>GAMVDKGFINIFPMINTTVFVNDGENVDLIVEYEAFP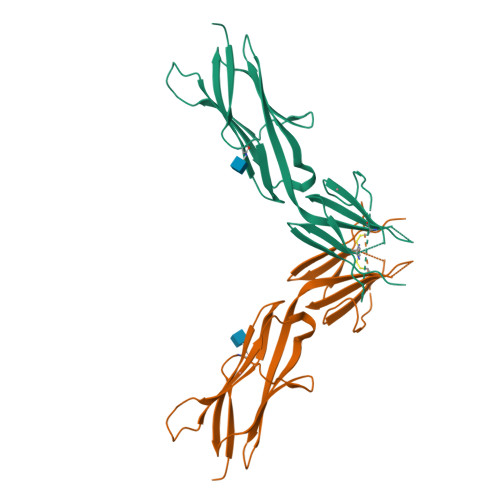KPEHQQWIYMNRTFTDKWEDYPKSENESNIRYVSELHLTRLKGTEGGTYTFLVSNSDVNAAIAFNVYVNTKPEILIRLVNGMLQCVAAGFPEPTIDWYFCPGTEQRCSASVLPVDVQTLNSSGPPFGKLVVQSSIDSSAFKHNGTVECKAYNDVGKTSAYFNFAFKEQIHP[3x]>MHNLQQLLPTRSLIWIFSFLTSISIWCTVAHAETEGRVQHFTGYIEDGRGIFYSLPDMKQGDIIYASMQNTGGNLDPLVGIMAEEIDPAVSLGQVLEKALASENDLISELTAVADRIFLGWDDDGGKGYSASLEFTIPRDGTYHIFAGSTITNQRLDKFQPTYTTGSFQLILGLNAPQVISGEGEPEGEVFASLASLEIKPEAHVQELEIRLDKDTRYLTQHTRNLQPGDTFHALVEPIGEAPLPRLRLTDSGGKPLAFGLIDQPGESVELNYTCDQDICELVVHVDGTDGQKDSGEAVYRLLVGINAPNLRESGQTPVGSSVFLESDLVTVGLAVDQIVGVDQRSENFSVVGTLKLSWHDPKLGFSPDQCGCTVKSFEDASIRAVAGEINLPLPSFSFYNQQGNRWSQNQVIFVTPDGRASYFERFTVTLQAPDFDFLAYPFDRQKFSIKVDLAVPTNMFIFNEIERFQQVVGDQLGEEEWVVTSYSQEITEVPFERGSTNSRFTTTLLVKRNLEYYILRIFVPLFLIISVSWVIFFLKDYGRQLEVASGNLLVFVAFNFTISGDLPRLGYLTVLDRFMIVSFCLTAIVVLISVCQKRLGAVGKQAVAAQIDTWVLVIYPLVYSLYIIWVYLRFFTDHIGW[5x]

Pentameric ligand-gated ion channels (pLGICs) constitute a family of receptors responsible for the rapid conversion of chemical to electrical signals in most kingdoms of life. To date, the only pLGIC in which an NTD has been partially characterized is DeCLIC, derived from a symbiotic sulfate-reducing deltaproteobacterium related to Desulfofustis glycolicus. The DeCLIC NTD accounts for roughly half the total receptor mass, and appears to accelerate activation and deactivation of the channel. Like several pLGICs, DeCLIC has been shown to be inhibited by calcium ions (Ca2+), mediated at least in part by a calcium-binding site at the ECD-TMD interface.

We then collected data in the absence of calcium, ensured by adding 10 mM ethylenediaminetetraacetic acid (EDTA) to the nanodisc-reconstituted sample. In order to identify potentially asymmetric conformations, we initially processed the resulting dataset without imposing symmetry, and identified two classes. Although both contained non-conducting pores similar to the calcium-containing structure, one of these (sym, 2.4 Å, 58 % of assigned particles) exhibited five-fold symmetry and was further refined with imposed C5 symmetry. The NTD density, albeit weak, enabled assignment of 87 % of NTD residues. Aside from the absence of ion-like densities in Sites 1, 2, 3, and 4, the sym calcium-free conformation was largely superimposable with the calcium-bound structure. The most notable difference in the absence of calcium was a local loss of definition in the density associated with loop F, indicating calcium may stabilize this region in a closed-pore state. Whereas no major changes were observed in the ECD-TMD regions in simulations with or without calcium, the NTD exhibited more flexibility, particularly upon calcium depletion. In simulations of the calcium-bound structure, the center-of-masses (COMs) of individual NTD1 lobes deviated up to 13 Å from their initial positions; in simulations of the structure without calcium (in the sym conformation), such deviations increased up to 25 Å. Similarly, NTD2 lobes deviated up to 7 Å with calcium, but up to 15 Å without calcium. Global properties also exhibited modest destabilization upon calcium removal: from an initial value of −26°, ECD twist varied in a 7° range with calcium, but in a 12° range without calcium.> AANDNNVEWNGLFHDQGPLFDNAPEPTSTQSVTLKLRTFKGDITSANIKYWDTADNAFHWVPMVWDSNDPTGTFDYWKGTIPASPSIKYYRFQINDGTSTAWYNGNGPSSTEPNADDFYIIPNFKTPDWLKNGVMYQIFPDRFYNGDSSNDVQTGSYTYNGTPTEKKAWGSSVYADPGYDNSLVFFGGDLAGIDQK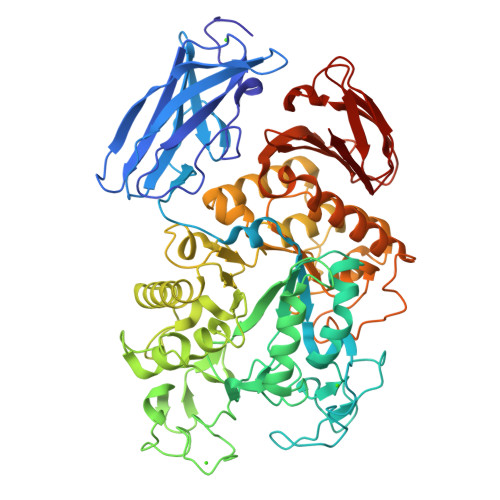LGYIKKTLGANILYLNPIFKAPTNHKYDTQDYMAVDPAFGDNSTLQTLINDIHSTANGPKGYLILDGVFNHTGDSHPWFDKYNNFSSQGAYESQSSPWYNYYTFYTWPDSYASFLGFNSLPKLNYGNSGSAVRGVIYNNSNSVAKTYLNPPYSVDGWRLDAAQYVDANGNNGSDVTNHQIWSEFRNAVKGVNSNAAIIGEYVGNANPWTAQGNQWDAATNFDGFTQPVSEWITGKDYQNNSASISTTQFDSWLRGTRANYPTNVQQSMMNFLSNHDITRFATRSGGDLWKTYLALIFQMTYVGTPTIYYGDEYGMQGGADPDNRRSFDWSQATPSNSAVALTQKLITIRNQYPALRTGSFMTLITDDTNKIYSYGRFDNVNRIAVVLNNDSVSHTVNVPVWQLSMPNGSTVTDKITGHSYTVQNGMVTVAVDGHYGAVLAQ>MTTGTEEARIPLDPFVTDLDGESARLRAAGPLAAVELPGGVPVWAVTHHAEAKALLTDPRLVKD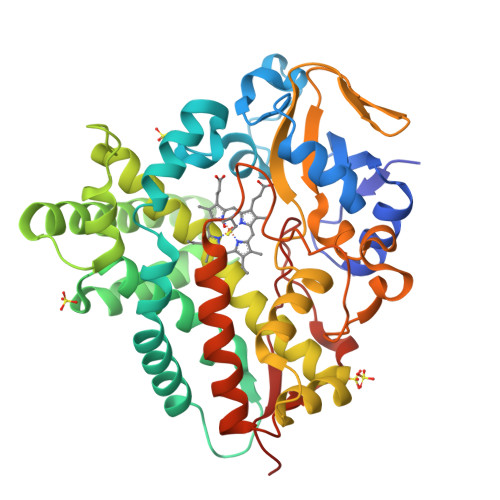INVWGAWRRGEIPADWPLIGLANPGRSMLTVDGAEHRRLRTLVAQALTVRRVEHMRGRITELTDRLLDELPADGGVVDLKAAFAYPLPMYVVADLMGIEEARLPRLKVLFEKFFSTQTPPEEVVATLTELASIMTDTVAAKRAAPGDDLTSALIQASENGDHLTDAEIVSTLQLMVAAGHETTISLIVNAVVNLSTHPEQRALVLSGEAEWSAVVEETLRFSTPTSHVLIRFAAEDVPVGDRVIPAGDALIVSYGALGRDERAHGPTADRFDLTRTSGNRHISFGHGPHVCPGAALSRMEAGVALPALYARFPHLDLAVPAAELRNKPVVTQNDLFELPVRLAHHHH[2x]> MDKEIYCGSVPVSYFDPFDLFESLRPEFQQILPLDNIHWKAFDGTVRTVNRLPIELIPEGRGEADKSNDEQPFIRFLIVNCISIDQYRAKVRPLVRQWLPNLESVSSSTGEKMIYKPIILLYANSEVVDSNLFKSVSLMEKFGKDFPHVQTLEVRSVYRSPKERQEFWNQFSQKIKASVLSIFQKRLTHLQHSLANLQKGNNFEEQLLTREKLYELYVVFNILEDASLELQKIKKEILRRNMNMPDGKLQVPFESSSKSDESLGSIIIEGTLDKFQLHKYFFIRRLRLLKLEDQTLTAFVGAFQLIKNFIESISIEYRKSVRLLEFKHYFITSMLSYFEFENVSNPLLCEIKAELLMLKRDNWVQGVMATSGYRLMDKNYPNSDVKYKFDLLKETFVDETVFQENFLTLTKEILSLFNKCEGKRQRIVDILSIEIGLLYYQGKKYEEAVSLFLSCYEYYTQTNKNSIGLKILQVFIDSLSHCPKLDVLQIDGESVSASAVLTNAFLNILKLCKDNDSKEIWWKKFMDLQMKNNIHLMYPLDGLFEVTLNSKVHLARANVSAIEVNLKSYGFPEDISTKTMRLSLKNMGGD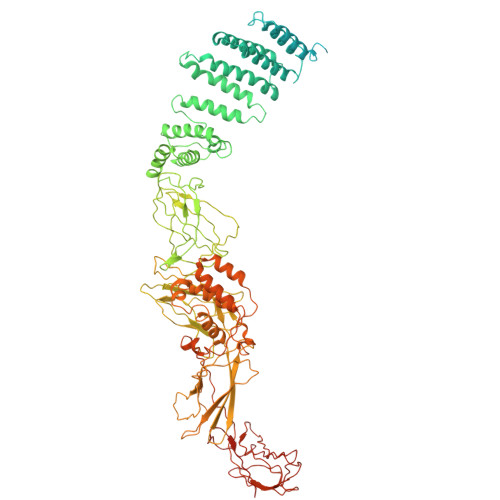VIVFGASDFLLKKGENKLILECRDIMYGEFSLLSFEIIVEGITFVKEFPENQDEFIVVPEIYCKESTKVLVKQAHNLNLGEYALELKSVQSDALESLQVEVEVQKNIGNMKNLPVSFSMDEIQARKRYNTPFENVRLEYYLLDQITAFDLIIKTSFTKKNDQGTFGETKKVRIQCYLQLSVSVEDIFKKDIFFFKFLLNSSVREEPVILYSSELSAPDTRNDYNIRGDYIATTPALITFDGNESFINCYEITANNNFDSKDIFNLKVRYNTLKEQLDCFITDAVLIEGDVEWFILFEKWKTFWELEILKKLKYDYDAFKENRIIRLLKTSIDLNKTKSKIRNLCIEKAVLDKILICLNKVSRGIAVCNTDMDEYVRNLVPKQLTVPVQLPGFEQFFHVQFEQMETSHDALHDTIATIGNSLSYTVIVENLSGQWGQDVIDDGGYIFEILSSNEWLIHGQKRCAIKEKRKEFEVHLIPLKKGYLNFPRVEITNINGKSCRVDHSNAFESILIF> QPNVDMGFEAAVAKKVVVPITFMVPNRPSGLTQSALLVTGRTFLINEHTWSNPSWTSFTIRGEVHTRDEP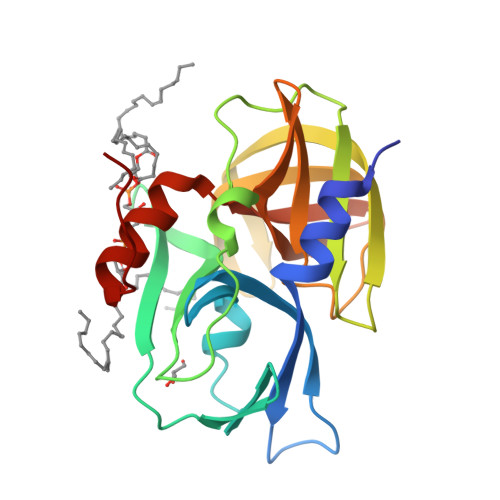FQTVHFTHHGIPTDLMMVRLGPGNSFPNNLDKFGLDQMPARNSRVVGVSSSYGNFFFSGNFLGFVDSITSEQGTYARLFRYRVTTYKGWCGSALVCEAGGVRRIIGLHSAGAAGIGAGTYISKLGLIKALKHLGEPLATMQ> HMLSDEQMQIINSLVEAHHKTYDDSYSDFVRFRPPVREGPVTRSASRAASLHSLSDASSDSFNHSPESVDTKLNFSNLLMMYQDSGSPDSSEEDQQSRLSMLPHLADLVSYSIQKVIGFAKMIPGFRDLTAEDQIALLKSSAIEIIMLRSNQSFSLEDMSWSCGGPDFKYCINDVTKAGHTLELLEPLVKFQVGLKKLKLHEEEHVLLMAICLLSPDRPGVQDHVRIEALQDRLCDVLQAYIRIQHPGGRLLYAKMIQKLADL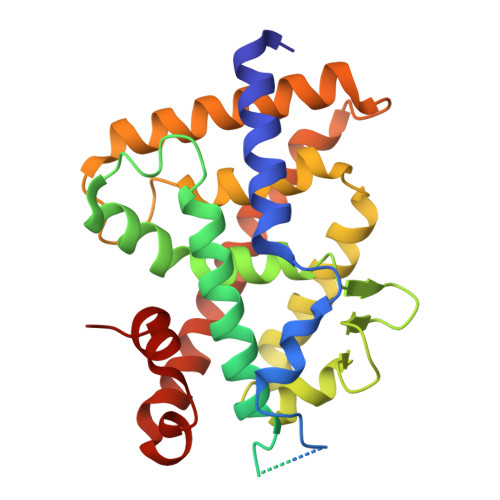RSLNEEHSKQYRSLSFQPEHSMQLTPLVLEVFGSEVS>[2x]STIEYNEILEWVNSLQPARVTRWGGMISTPDAVLQAVIKRSLVESGCPASIVN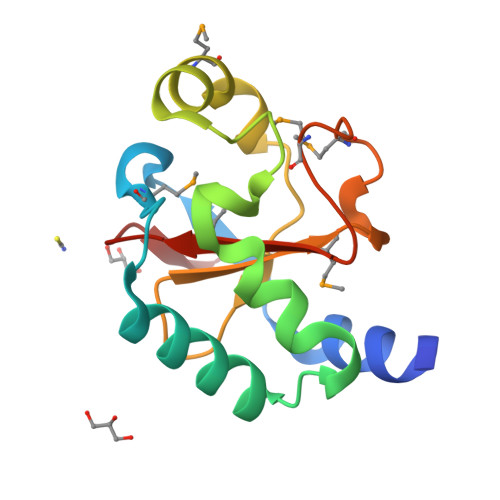ELIENAHERSWPQGLATLETRQMNRRYYENYVAKRIPGKQAVVVMACENQHMGDDMVQEPGLVMIFAHGVEEI>[9x]MTDTHTGPTPADAVPAYPFSLPHALDLDPHYAELRRD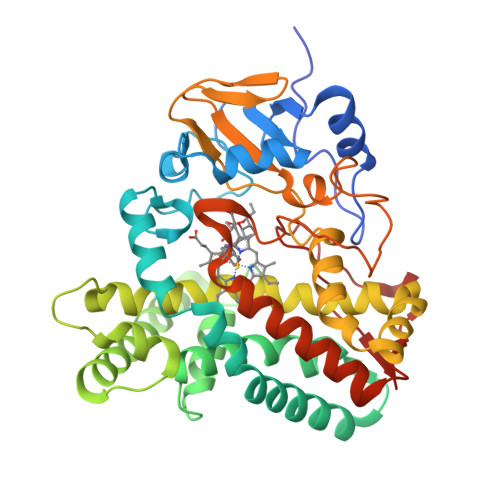EPVSRVRLPYGEGTAWLVTRMSDARIVLGDSRFSTAAATDPATPRMFPTPPEPDGVLAQDPPDHTRLRRLVGKAFTARRVEEMRPRVRSLVDSLLDDMVAHGSPADLVEFLAVPFPVAVICELLGVPLEDRDLFRTFSDAMLSSTRLTAAEIQRVQQDFMVYMDGLVAQRRDAPTEDLLGALALATDNDDHLTKGEIVNMGVSLLIAGHETSVNQITNLVHLLLTERKRYESLVADPALVPAAVEEMLRYTPLVSAGSFVRVATEDVELSTVTVRAGEPCVVHFASANRDEEVFDHADELDFHRERNPHIAFGHGAHHCIGAQLGRLELQEALSALVRRFPTLDLAEPVAGLKWKQGMLIRGLERQIVSW> KLGKLQYSLDYDFQNNQLLVGIIQAAELPALDMGGTSDPYVKVFLLPDKKKKFETKVHRKTLNPVFNEQFTFKVPYSELGGKTLVMAVYDFDRFSKHDIIGEFKVPMNTVDFGHVTEEWRDLQS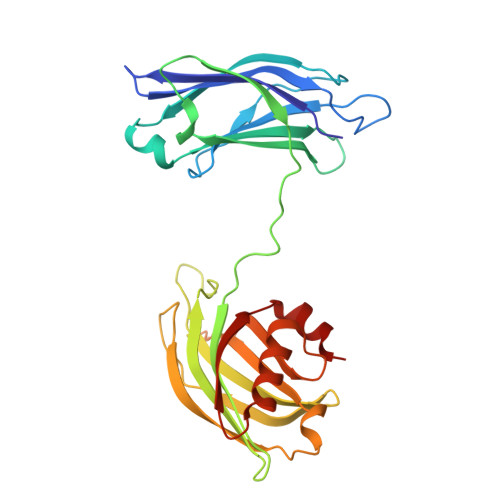AEKEEQEKLGDICFSLRYVPTAGKLTVVILEAKNLKKMDVGGLSDPYVKIHLMQNGKRLKKKKTTIKKNTLNPYYNESFSFEVPFEQIQKVQVVVTVLDYDKIGKNDAIGKVFVGYNSTGAELRHWSDMLANPRRPIAQWHTLQVEEEVDAMLAV>ENSVFFGKKKKVSLHLLVDPDMKDEIIKYAQEKDFDNVSQAGREILKKG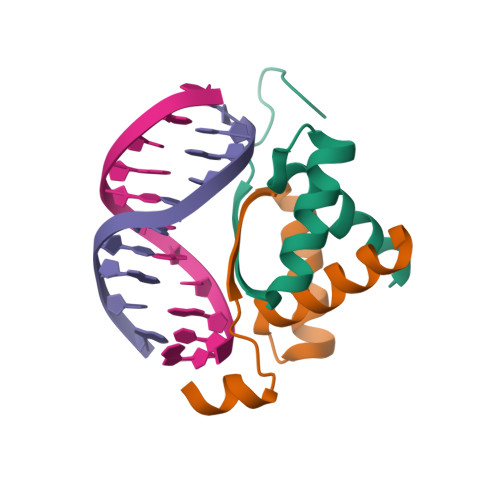LEQIA[2x]> MSEVESQQSQETNGSSKFDVPEIELIIKASTIDGRRKGACLFCQEYFMDLYLLAELKTISLKVTTVDMQKPPPDFRTNFEATHPPILIDNGLAILENEKIERHIMKNIPGGYNLFVQDKEVATLIE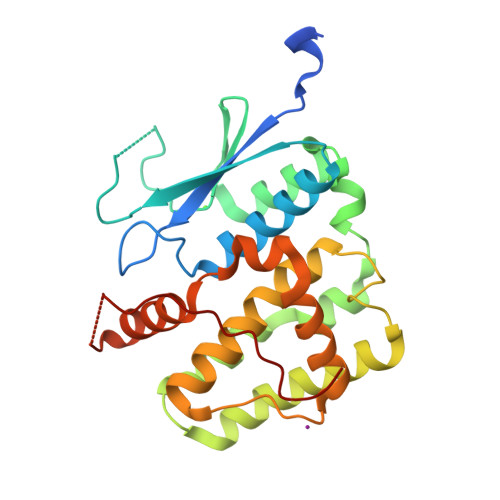NLYVKLKLMLVKKDEAKNNALLSHLRKINDHLSARNTRFLTGDTMCCFDCELMPRLQHIRVAGKYFVDFEIPTHLTALWRYMYHMYQLDAFTQSCPADQDIINHYKLQQSLKMKKHEELETPTFTTYIPIDISE However, the parasite also displays members of variant protein families on the surface of infected erythrocytes, including the multidomain Plasmodium falciparum erythrocyte membrane proteins 1 (PfEMP1). These PfEMP1 cause infected erythrocytes to adhere to the surfaces of blood vessels and tissues, removing them from circulation and protecting the parasite within from spleen-mediated destruction. ICAM-1 binding is mediated by a subset of Duffy binding-like (DBL) domains, the DBLβ domains, which are found in either A-type or BC-type PfEMP1 (26–29). To understand how these BC-type PfEMP1 interact with ICAM-1, we have determined the structure of the DBLβ domain of the B-type IT4var13 PfEMP1 in complex with the N-terminal domains of ICAM-1, revealing divergent, but similar, modes of ICAM-1 binding across the PfEMP1.

The IT4var13 DBLβ domain interacts with domain 1 and 2 of ICAM-1 through a complex binding site, the location of which is compatible with a previous study, and binding is mediated by 3 types of interaction. A major part of the interface is mediated by hydrogen bonds, contributed by DBLβ domain side chains from a central loop (residues 973 to 976) and helices in the C-terminal third (subdomain 3) of the domain (residues 1098 to 1121). All of these DBLβ side chains targets the backbone of ICAM-1, with the exception of glutamate 1098, which forms hydrogen bonds with arginine 49 in ICAM-1D1. Secondly, a loop from the DBLβ domain (residues 1107 to 1117) interacts through backbone–backbone hydrogen bonds with ICAM-1D1 to add an antiparallel β-strand to the A′GFC β-sheet of ICAM-1D1. Such β-strand augmentation is a common motif in protein–protein interactions but has not been observed in other PfEMP1–receptor interactions. Finally, the interface is stabilized by a cluster of hydrophobic residues found on an elongated helix of the DBLβ domain and 2 subsequent loops (residues 1102 to 1139). This cluster complements a hydrophobic patch on ICAM-1D1 which has previously been identified as important for ICAM-1 binding by B-type PfEMP1 (27, 35, 36). In contrast, mutation of 3 of the 4 hydrophobic residues that contact ICAM-1 (L1102, I1106, and F1113) reduced the interaction affinity by more than 200-fold, highlighting the importance of this hydrophobic patch for ICAM-1 binding. However, the B-type binding site is more compact, and the overall structure of the DBLβ domain in this region is more similar to that of previously characterized non-ICAM-1 binding domains. An overlay of the 2 structures, based on the DBLβ domain, shows that, while domain 1 of ICAM-1 is in a similar position in both structures, the protruding A-type ICAM-1 binding site fixes the C terminus of domain 2 at an angle that is ∼30° different from the position that it adopts, relative to the DBLβ domain, when bound to the B-type IT4var13.

> PCVVGGQADTIYPAIANQMAHQMHEDAQTEASKRGLAKLRADAKQGIYKKNRKPQELSNICNITLQHSNDSRNGNNGGACTGKDGNNERFKIGTEWKIGEKVETTDTDAYIPPRRQHMCTSNLENLNVSWVTEDGKAIHSLLGDVQLAAKMDADEIIKRYKKHNTLTDPIQQKDQESICRAVRYSFADLGDIIRGRDLWEHGDQTKLQGHLQIIFGKIKEEIKKKHPGINGNDKYKGDEKNNPPYKQLREDWWEANRHQVWRAMQCELKNLKKSNGDCHYNSRGTPLDDYIPQRLRWMVEWAEWFCKMQSQEYDKLMKQCSQCMSKGGDCRKGDVNCTSCEQACEEYKKKIKKWEKQWNKIKDKYEELYLQAKIAFAGTSFGGGDRDYQQMVHFFKELQKVTGDTTLGDTTSPYSTAAGYIHQEGHVDECTEQTQFCKNRNGNTASGKEDDNYTFKDPPPKYANACKCD;> QTSVSPSKVILPRGGSVLVTCSTSCDQPKLLGIETPLPKKELLLPGNNRKVYELSNVQEDSQPMCYSNCPDGQSTAKTFLTVYWTPERVELAPLPSWQPVGKNLTLRCQVEGGAPRANLTVVLLRGEKELKREPAVGEPAEVTTTVLVRRDHHGANFSCRTELDLRPQGLELFENTSAPYQLQTFG> SGIVPQLQNIVSTVNLGCKLDLKTIALRARNAEYNPKRFAAVIMRIREPRTTALIFSSGKMVCTGAKSEENSRLAARKYA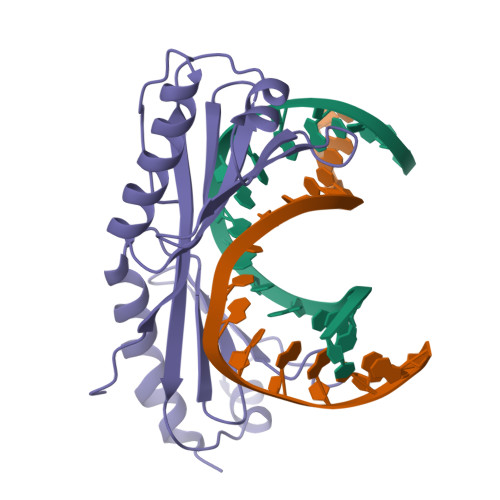RVVQKLGFPAKFLDFKIQNMVGSCDVKFPIRLEGLVLTHQQFSSYEPELFPGLIYRMIKPRIVLLIFVSGKVVLTGAKVRAEIYEAFENIYPILKGFRK> PKYDLFKPLDFLACVKSVHVAYHPGRPRSEVCRQLIHHMKSDS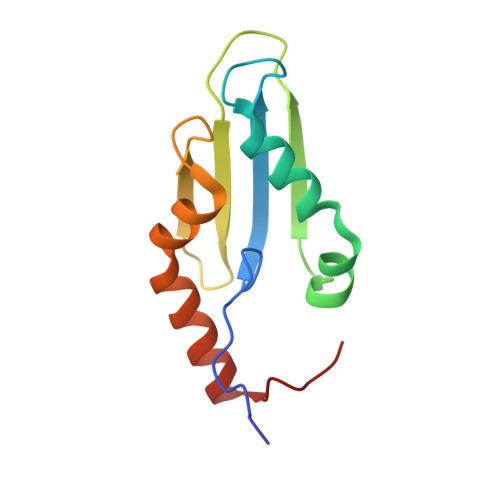VRKRFPSLQASYQLLGYNAPSTIKIELINGKKHEFQAEHFSLREMQMRFDTDQFEAYLEYMKSQSVEAKP Bacteriophage E217 infects Pseudomonas aeruginosa and is part of an experimental phage cocktail developed to eradicate P. aeruginosa infections in Galleria mellonella (wax moth) larvae and vertebrate models. E217 is a PB1-like Myoviridae of the Pbunavirus genus characterized by a ~66.2 kbp genome, significantly smaller than the classical enterobacteria phage T4 (~169 kbp). Here, we describe the structure of the whole E217 virion before and after DNA ejection at 3.1 Å and 4.5 Å resolution, respectively, determined using cryogenic electron microscopy (cryo-EM). We identify and build de novo structures for 19 unique E217 gene products, resolve the tail genome-ejection machine in both extended and contracted states, and decipher the complete architecture of the baseplate formed by 66 polypeptide chains.

We defined the atomic structures of all neck components, namely the head-to-tail, collar, and gateway factors, which connect the icosahedral head to the contractile tail. The first part of the E217 tail, or neck, was visualized in a localized reconstruction after applying C12 or C6 rotational averaging, which yielded maps at 3.3 and 3.4 Å resolution (FSC = 0.143), respectively. One unique penton of the E217 capsid is replaced by the dodecameric portal protein gp19, which is an attachment point for the ~1500 Å tail apparatus. However, unexpected for a Myoviridae, the E217 portal also contains a C-terminal α-helical barrel projecting into the head. Interestingly, the barrel is folded only in the pre-ejection conformation when DNA fills the capsid. E217 portal dodecamer is attached to twelve copies of the head-to-tail factor gp27, which closely resembles P22 gp437. Gp27 assembles to the portal by inserting its extended C-terminal tail at the interface generated by two portal subunits, suggesting the head-to-tail factor oligomerizes upon binding instead of existing as a pre-formed dodecameric ring. The other two neck factors, gp28 and gp29, reduce the C12 symmetry found in the portal and head-to-tail to sixfold, which is maintained in most of the tail apparatus. Six collar proteins pack under the head-to-tail dodecamer with gp28 N-helix positioned orthogonal to two gp27 subunits, explaining the C12:C6 symmetry mismatch. The last neck factor, gp29, connects the neck to the sheath lattice.

>[6x]IPGANLLRMAFGVIGTQIVRYRKFEQRVKNDQAQYVSMFGEPFDLAASVQRVRRDQYAQFNLEFQRNYVMIFANFDMVDLDRNMAGDQFLWTGRVFQLESQGSWFYQDGWGVCLAVDIGAAKA;>[12x]MVIFDEHKFRTLFPEFADPAAYPDVRLQMYFDIACEFISDRDSPYRILNGKALEACLYLLTAHLLSLSTMQVQGAAGGGVTAGGTQGGFITSATVGEVSVAKLAPPAKNGWQWWLSGTPYGQELWALLSVKAVGGFYIGGLPERRGFRKVGGTFW;>[6x]MFDGELIAKLVVELNAAMTSAQEALQFPDFEVVQKAQPTQQGTSTRPTIFFQKLFDIPRGWPATDWHLDNTARKYVEITRQHVETTFQISSLHWQNPEITHVVTASDIANYVRAYFQARSTIERVKELDFLILRVSQISNEAFENDNHQFEFHPSFDMVVTYNQYIRLYENAAYSADGVLIG;>[12x]PTMLQDWYNSQGFIGYQACAIISQHWLVDKACSMSGEDAARNGWELKSDGRKLSDEQSALIARRDMEFRVKDNLVELNRFKNVFGVRIALFVVESDDPDYYEKPFNPDGVTPGSYKGISQIDPYWAMPQLTAGSTADPSSEHFYEPDFWIISGKKYHRSHLVVVRGPQPPDILKPTYIFGGIPLTQRIYERVYAAERTANEAPLLAMSKRTSTIHVDVEKAIANEEAFNARLAFWIANRDNHGVKVLGIDEGMEQFDTNLADFDSIIMNQYQLVAAIAKTPATKLLGTSPKGFNATGEHETISYHEELESIQEHIFDPLLERHYLLLAKSEEIDVQLEIVWNPVDSTSSQQQAELNNKKAATDEIYINSGVVSPDEVRERLRDDPRSGYNRLTDDQAETEPGMSPENLAEFEKAGAQSAKAKGEAERAEAQAG>[2x]MSERLSITPLGPYIGAQISGADLTRPLSDNQFEQLYHAVLRHQVVFLRDQAITPQQQRALAQRFGELHI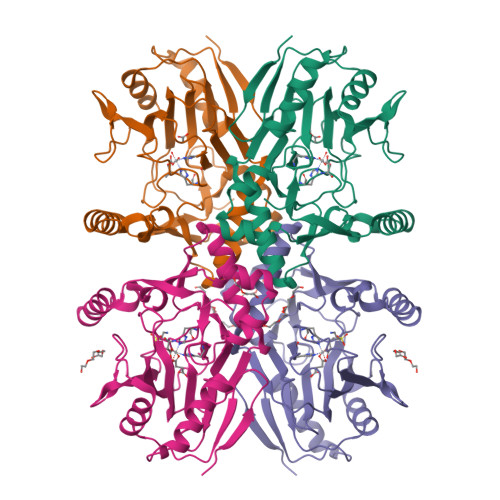HPVYPHAEGVDEIIVLDTHNDNPPDNDNWHTDVTFIETPPAGAILAAKELPSTGGDTLWTSGIAAYEALSVPFRQLLSGLRAEHDFRKSFPEYKYRKTEEEHQRWREAVAKNPPLLHPVVRTHPVSGKQALFVNEGFTTRIVDVSEKESEALLSFLFAHITKPEFQVRWRWQPNDIAIWDNRVTQHYANADYLPQRRIMHRATILGDKPFYRAG> GDVVEAIEGAVARVADTISSGPTNSQAVPALTAVETGHTSQVVPGDTMQTRHVKNYHSRSESTIENFLSRSACVYMGEYYTTNTDETKRFASWTINARRMVQMRRKLEMFTYVRFDVEVTFVITSKQDQGTQLGQDMPPLTHQIMYIPPGGPIPKSTTDYAWQTSTNPSIFWTEGNAPPRMSIPFVSIGNAYSNFYDGWSHFSQNGVYGYNTLNNMGQLYMRHVNGPSPLP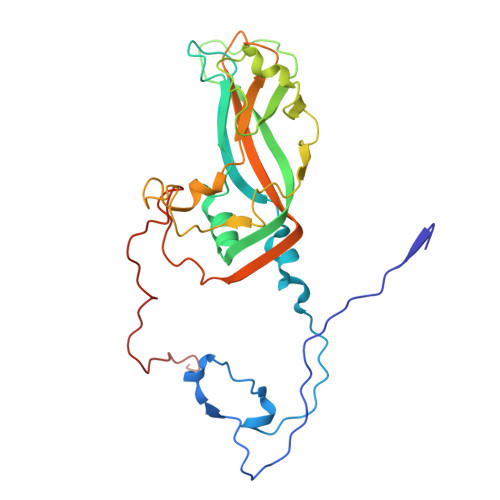MTSIVRVYFKPKHVKAWVPRPPRLCQYKNASTVNFSSTNITDKRDSITHVPDTVKPDVTTH> GQEQAKVWTQTARANAEKNNAQLSTLLTDDQIGAIYGYTTNEGYTALNPALRGQTPLTPELEAFTGHVTDGLNKLPAYNGETYRGTTLPAHILEQNQIGGTVSDGGFMSTSAKTPFDGDVSISVRGNSGKQIDFLSKYKNEAEVLYPPNTRFEVINRIE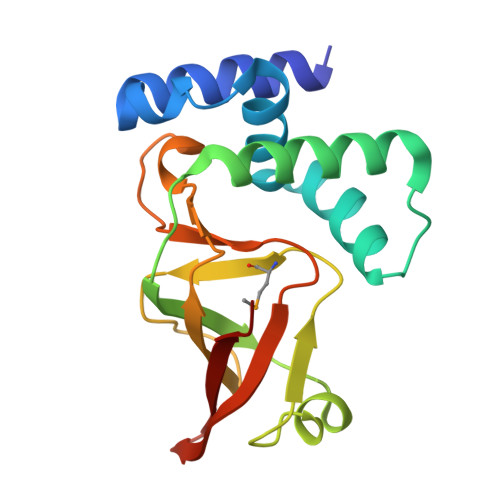QNGTTHLLYREIP ERYTHOSE-4-PHOSPHATE | C4 H9 O7 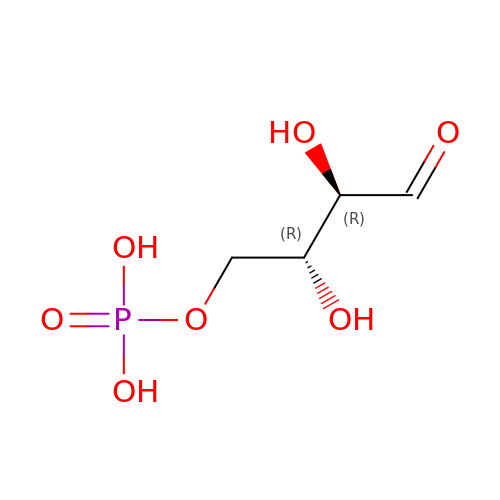P | NGHMDNPXVRFFGS-IUYQGCFVSA-N> MAASSPLVRLRRLALPLALVVLCAAAAHGQTLSSAVLTASNTIMATLSNVTTSTDCRAAFAYFDSNNATKAASPFANCTVSGTTSVTLILASGVSYAAGDQLNIKVNQTTLNTTAGVPFVPAAAAAAVQPVLGAATLTTASSLVVKLPLSSGNTMPDGYATNMTICGAAVQLLSAAGAVKASPFSACLLAADTLTLTLTSSGTYAPGDVVNVVAGQSTLKNGATSYTKSAAGSVIRPTLTTVSLATTTTILIGASAPVSLPANASADVCNSIFTVALKSGTALPTALSACMAGPAVTAITATFANGTTYSDGLTVTIKANQTLLRTGDQSASSPLFLPPASALVIAPTVLSASLTSATSITVQLPVSSTASGTLDAAGCNGAFELRAAGSSASKSSPFSACALASNNTALVLTLASASTYTAGDIFNVKSGQSLLQVGSTAYVPQAVSVLPTLSTAILVAASVVRVGLPVVSSIPAPYSADDCARSVIIAAANSTAAKAISGCVLSADGKALLVTLGAAYAAGDTVNVRTGQWQLRAGASVTLGPNYIAASTPVAIVPGFSSAVLTSATQVTVQLPLASALPATISASECGDAFDLLDASGTTSRVSPWTGCSIGSNNTLVLNMTAGIYVVGDQVTPKSGQTKLTFANTTAYGVLLTPINPILTAATTAMLTASSTIVVALPYAANLPASTNNGTVCNAAFDLVSAAGASRTAPFSACSISGGTTLTLTIASTASYTAGDRINVKSGNSAFLGSLSASGPAFVHAGTAIVITPTVVSTALISNTNVFVSLSAPTSASAFNQSICNGAFDVSGLATPFTNCTLSADGTGISFLLASAGSVTSGVTTINVKSSQLFLLAAGSGSSDSPAFVPRGSALTISEAKLAGAYLTAANTIIVKLSVAAAAVDGFSSSCNNVFTLFNSSGTARASPFSACTLSTDGLTVTLTTSSWVSTDKLNIRSDQTLLKVLGAANGPSYPALSSATEVSPAITSAHITSPTTIIVPLPVASDLTGSSCSFLVLTAATSNCALSNNGTLLTVTLSGSYTIGDTININALNSALRGTSSTGALYQPVSGATAATIQPTIGAVQVTTSTRLLVTLPAAMSSPVPNPLTADACNAALDLSGKSSPFAACTASGTTLTLDLASAFVPGDRLNVKSTNTALRLGTGASALFFQPLATSPANILNPTFVSAKATSTSVVVVSLPAASTFVKSGSATAGLVKADCDTVLAMSSGSLVGSGNACDLNTTSSSQLIVTLAGTTYAPGQTINVLTTNTMLLAGSSSGPAYQPRTITINPAYLSSDVVATAPDTVVVTLPVTSGLFAADGSSLGSTLTAAQCATVLEVKAGTTAKGLASCSLAGTTLTVKLLGNNSDVYTGGDTFNFKDTNALLLAGSANTAPAYKALATAAVIVPNLYKAVASAGDTILITLPAASTFVVSGSAVLSVSDTVCNTILTFTNSKTVKSGTNCVITGAVLSLTLNSAITDQTTVTINSGGQTTLVSGTGTTGPAYKAGTAAPISPAYLTSAAARSATSIVVTLPFTSTVNGATLTKATCDTIVEVLNGGDATKPRTLDSGTPCTLATTLLTVNLAATESFAPGDTVRIKSGNTVLLIGSAGGNAPYVQATTATPIALGYVTSSIATKATEIKVTLPVPITLIKAGVSVASLDKTDCDTLLTVASGTLAATGSCALSGTVLTITTTSTYTPGTTTVQFTAVASSASVKILGGAGTTGTIIAALSAASSVLPGYLTSAVISGANTFTLTLPYAVTSGGNPTCSDIIEIKAANGAMKTFNGVCSVASATTVTGTTNEALLASDTVTLKGAQNALTTTTGSKIYAATAAINIQPAYLTGAYAIDDKKFVVVLPYASTLAAGTCSSIVSVTDNNNGPAESGCSLALDGTGIYLTVTVSASLTATAWKVDFKAAQTALTVGSTAWAPMATGTAKSLNAGATTWGSSIMTATAVATNVLEVTLPMSSYMADISSGCSPVTFSTANTAASCKLIGTTSSPNSILQITLTAGYVAGAVSLANAAGLIKAGSASGTAIGAASTVTIKPTFVSAVATGPRTIVVALPIQSKIIKGAPTCTGGAVTCSSGTATCQSGSPACSAAGTYTCTATDPTVGLTCAAPTVTCPASTTAACITGGSPGSIATAGNGPGCAAATTDGGTAACGAGISAVCYSSSLTTAARCASGSAFSAANGNNCDDSASSIDLDPTCYTSSTMTATAVSDAALCTGWISGMPTCSSSGKFACVSATGPTCTASTAPTCKSPFTGTANCAITFSCGGTGLVVPTCTGSFTGCSKGTTGDTCDDDIASPADCSTIFSLTGGTATIAGCSNPGSDFTAPYTTTVTLATANWVPGTTLSVAADQAAAAATNYLKPTAAITLLYTTKPSGAVVIYPSISSATLTGPKSLQVTLPVAASVPSSGLSPADCNNIFQLYATGTTTPKTAAVFSACYLGADKQTFYLTLAAAAASTTNANTYAVKDLINIKAGQSLLKADSATAANRLAFAPLPDALLIRPAITSAVATTIASAAVIKMQLPLTSNLGTVNCATTGIKVRVDDATDKTQANTGACSISSDANGAVLTLTLNQALGASDFTTGKGVSVVVVATSSADATKLQLFGGSDNTGPLYVTGSIPVYDVVTPGQSIVSAKAIASNQVEIKLPAPSTITTGNTCANFLAFTPTRTISSCVYDAETQLVTATVDQFAAGDAVNIAGAPNLLKYATAAATLTDYAALAAAATVSPALVSAYTVDSTTIAVVLPATSSFYSGATNSATKVASLTDVECADVLTVLLAGKTNSAGVSACATPSNCRTLFSGAACLLGTTSAGDTLLTIKLGASYAAGDAVDVWDKNAGLNGATAAAKPLRVGTNVQALYVPRRMPVVIEPRIVSASATGARTIAVTLPVTSQLIDSTGTVISAPTQQQCASLVALPAGKSVASCAISSDFLTLTLTLAADFAPGDTVNIASGQTLLRAWKSDVGPGYELSGPLYTPSASAVTVTLSFFVSATSTAANTIVVTLPFPVKMYDLAASPAEILAADGATPTKDNCDSVIRVIPSGSTIARTLVAPGAGVAPCVLSGSGTTITLTLDTTVSSYATGDRIDVGFGNSANLRGAATAAAVANTSPKYTTVATLNAAASAAVVTIGPSIVSAAAASPTQVKVTLSATGTITTTPATVDDCNKIVTFTPAKTLAATSPCSVAGTTLTVNLDKATPYAGTDAVNIAAANSLAATTNPLKAGSLAFVAKATAVTIDPNLYTATAIDSLVYEVALPAASSVGSTALTAAQCGAILSLTGGRTISSTVTAPCVLDTTKTLLTVSLGTAYADGDTVTLQSTQATPWLRAASDTGPAYKVGSTLIVKPTIASAKATTATTIEVTLPVTSVIWSTSGGAAVSTALTATECGKILSVKRGSGTVALSASGACSLSSSGSTTLTVTLASDQVFQAGDKINILASNTDSANTDKYLVATTSSSGQAYIARSSDVVIAPGFINAAYAVGPNTLSVALPVVSSIATDNDCSTVVTVRASATPTTTRTVSGACTVASDATGYYLVVTLAAGTPFVSGDEVLIKSGNTALVGSIAYASGAAGATKPIYANFDDAILTAPTTVLVTMAAVTTVSFTSKADCDAVFVFSGAGNTTKTTSPIASCALAPDGLSVTITLSSADAYVPGDAINVVKDQTSAKVGGVGGTNLVPYPTATTISPRPFGAKATLVAPTSVAFSLPAVSSLPAATAAADCNAAVRYTDVAGVDAVNPFTSCALTPDTKGVVLNTASPIYKAGDVMNIKSGNAAVRWGPQASGAAYYPAAADVPVFATVATATLVDPSTVVLNLPTVSAIPDNFTVPDCLRAIEFKTAAGVTKNGTVASCMLMPDRLGLQVKLLSAGNFSAGDTVNIKPEQAELRSSALATGPSYVPKLAAQVVNPALFANANLTSATAITVRLPFASALATGADCKAVLALLGAGGVAKNVSSCSLGADGVTLAVTIPAASFVGGDVLNIVPGQRALTLADGTTAYVPSKAGVLVTPNIVSATLTNATIVTVALPTASVLTSTAAADCNAAVVIARNGSAVASPLSACAVSADGLSLTLTAAATYKPMAGDTVDVAVSQTVLRAGSATGPAYVPRPSPALITVPSPPPSPPPSPAPSPPPSPPLSTANYSARGLATGPLSCNVLIGDLTVTTTAGNFTTIGMASYAGKDASYKGSCKDAVTGAVYTDDTVASTLPAGLTGLVLSPVTALASVWDLKSVADLANTNKDYLRLFGVPVNASAYGTAVQLLAYDYYVKGFVALETPAVAVLNVEGMVAANLLMYTKFFDGLNTSVAGRDITAAQALAAGQYALAAVLEDSIAPINTTDPASILALLNVTYSVLTANATSAAGRRLLQTAPAPFTQLQAQATALAAAAAGSNALVAAQQARLITAINAGTSISAAELTNIINEASKVIVAQSTVIATAATGLGSGAISPASFTSSYTGSALSTLVAQQQLAATPGSDVTAGPAPSPPSDKKKSNTGLIVGLVVGLVGGAIVITLIVVFIVMRRRKQNVAAAGQATA

Bloodgood and Sloboda have shown that the flagellar membrane glycoprotein 1B (FMG1B), an unusually large ≈4546 amino‐acid long molecule, constitutes a major part of the glycocalyx of C. reinhardtii, which localizes to the ciliary coat and is visible as a densely stained layer in electron microscopy sections. FMG1B is described as a mucin orthologue which lacks the major O‐glycosylation of mammalian mucins but is N‐glycosylated. The results find FMG1 to form a protective layer with adhesion‐regulative instead of adhesion‐conferring properties and an example of an undescribed class of mucins. In wild‐type cells, the ciliary membrane that surrounds the central axonemal structure is coated with a diffuse inner layer of low electron density and an outer, electron‐dense layer consisting entirely of FMG1.

Instead, we purified FMG1B from C. reinhardtii cilia by concanavalin A affinity chromatography and performed single particle cryoEM analysis. The resulting ≈3 Å structure of FMG1B revealed the molecule as a long, twisted chain of 34 individual globular subdomains of 109.6 ± 10.9 amino acids and one cysteine‐rich coiled domain. The individual subdomains fold into an Ig‐like fold with each two orthogonal beta‐sheets and one short alpha helix, which we call beta chunk repeats (BCR). We modeled the semi‐rigid structures composed of the chained BCRs to high confidence, while the flexible nature of the cysteine‐rich domain resulted in a lower local resolution density which, together with the absence of bulky, recognizable amino acids, could not be assigned confidently. The C‐terminus of FMG1B consists of an ≈100 amino‐acid long intrinsically disordered region (IDR) linker followed by a multi‐helix transmembrane domain (TMD). Due to the inherent flexibility of the linker region, no densities could be resolved for either the linker region or the TMD. Despite the high sequence variability between individual BCRs, every BCR contained a single highly conserved disulfide bridge as confirmed by MS‐assisted disulfide detection, while no disulfide bridges were detectable in the cysteine‐rich domain under our conditions. Interestingly, we observe protruding densities by cryoEM that cannot be explained by the primary peptide sequence. Strikingly, we find a near‐perfect correlation between the identified candidate sites and the unexplained electron densities. As such, we were able to directly confirm 25 glycosylation sites of FMG1B, which were mostly located to the 16 n‐terminal and the 9 c‐terminal BCRs, all of which were in proximity to each other on one side of the FMG1B molecule.>[2x]MW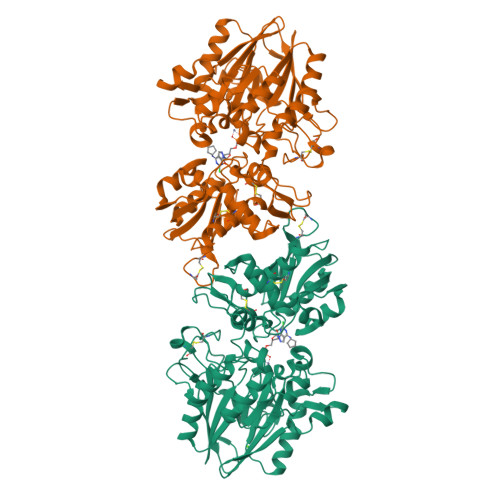ELTILHTNDVHSRLEQTSEDSSKCVDASRCMGGVARLFTKVQQIRRAEPNVLLLDAGDQYQGTIWFTVYKGAEVAHFMNALRYDAMALGNHEFDNGVEGLIEPLLKEAKFPILSANIKAKGPLASQISGLYLPYKVLPVGDEVVGIVGYTSKETPFLSNPGTNLVFEDEITALQPEVDKLKTLNVNKIIALGHSGFEMDKLIAQKVRGVDVVVGGHSNTFLYTGNPPSKEVPAGKYPFIVTSDDGRKVPVVQAYAFGKYLGYLKIEFDERGNVISSHGNPILLDSSIPEDPSIKADINKWRIKLDDYSTQELGKTIVYLDGSSQSCRFRECNMGNLICDAMINNNLRHADEMFWNHVSMCILNGGGIRSPIDERNDGTITWENLAAVLPFGGTFDLVQLKGSTLKKAFEHSVHRYGQSTGEFLQVGGIHVVYDLSRKPGDRVVKLDVLCTKCRVPSYDPLKMDEVYKVILPNFLANGGDGFQMIKDELLRHDSGDQDINVVSTYISKMKVIYPAVEGRIKFSLEHHHHHH>SHMEDYIEAIANVLEKTPSISDVKDIIARELGQVLEFEIDLYVPPDITVTTGERIKKEVNQIIKEIVDRKSTVKVRLFAAQEEL[6x]

CDFs are utilized by MTB to transport iron cations from the bacterial cytoplasm into the magnetosome lumen during nanoparticle biomineralization. Like most CDFs, the magnetosome membrane-associated (Mam) proteins MamB and MamM share a common two-domain architecture consisting of a trans-membrane domain (TMD) and a cytosolic C-terminal domain (CTD). Here we studied magnetite cluster MamB and MamM CTD structures from a phylogenetically distant magnetotactic Deltaproteobacteria species, BW-1 (MamBBW-1 and MamMBW-1). Each MamBBW-1 and MamMBW-1 monomer consists of two alpha-helices and three beta-strands and is folded like-metallochaperone, similar to previous CDF-CTD crystal structures.

To obtain structural and biochemical information, recombinant His-tagged MamBBW-1 and MamMBW-1 CTDs (residues 190–270 and 213–293 respectively) were over- produced in E. coli cells. SAXS results showed that MamBBW-1 scattering curves are similar at concentrations of 1 and 5 mg mL-1, indicating that the molecular dimensions are independent of protein concentration over this concentration range. In contrast to MamMBW-1, MamBBW-1 crystal structure exists as a monomer and does not create the classical V-shape dimer in the crystal, yet superimposition of MamBBW-1 monomers over MamMBW-1 V-shape dimer implies that MamBBW-1 may in high probability form a V-shaped dimer under the right conditions. MamBBW-1 dimerization interface, similarly to all CDF-CTD structures, showed the typical parallel S-shaped backbone structure. Support for such dimerization can be found at the possible interaction between Val235-Pro231 and Ile233-Thr234 from each monomer. Additional support is given by the MamMBW-1 and MamBBW-1 electrostatic potential maps, showing that the top of MamBBW-1 monomer and the top of MamMBW-1 V-shaped dimer have hydrophobic and positive patches, while the lower parts have hydrophobic and negative electrostatic charges. As an alternative, MamBBW-1 different oligomeric state can also be explained by crystal contact and crystallization conditions that break the dimer and create alternative contacts with similar or lower energy. Putative BW-1 C.B is composed of Glu271 (MamMBW-1) or Glu224 (MamBBW-1) from each monomer. Trp269, Val307 (MamMBW-1) and Glu222, Lys260 (MamBBW-1) are also located at the hypothetical metal-binding site but are not predicted to be involved with metal chelation. Overall, based on our analysis, it can be assumed that the composition of amino acids within MamBBW-1 and MamMBW-1 putative metal-binding sites are suitable to coordinate and bind metal ions.>[2x]GSSMCRAASLLPGTWQVTM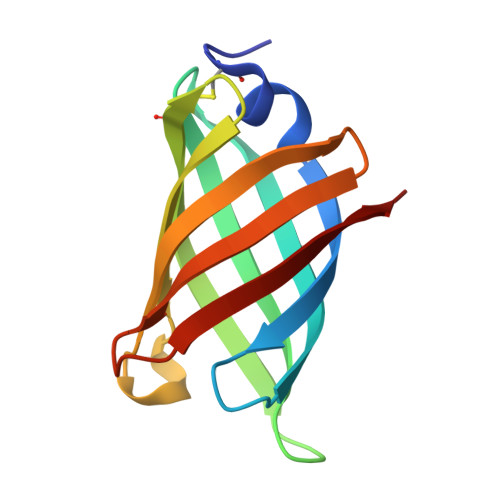TNEDGQTSQGQMHFQPRSPYTLDVKAQGTISDGRPISGKGKVTCKTPDTMDVDITYPSLGNMKVQGQLTLDSPTQFKFDGTTSDGSKLTGTLQRQE>SNAMKMSELEKMLKGEHFDGASAEIEALRSQAGRLKLEINQSLDEAERYALQRELFGHLGHKSCVQPPFHCEFGKTIRIGDHTFINMNVVMLDGAPITIGDHVLIGPSTQFYTASHSLDYRRRQAWETICKPIVIEDDVWIGGNVVINQGVTIGARSVVAANSVVNQDVPPDTLVGGTPARI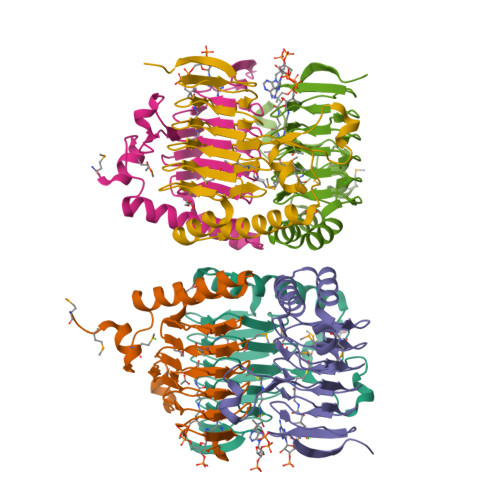LRSLKDPAESMAE[12x]> QWALEDFEIGRPLGKGKFGNVYLAREKQSKFILALKVLFKAQLEKAGVEHQLRREVEIQSHLRHPNILRLYGYFHDATRVYLILEYAPLGTVYRELQKLSKFDEQRTATYITELANALSYCHSKRVIHRDIKPENLLLGSAGELKIADFGWSVHAPSSRRTTLAGTLDYLPPEMIEGRMHDEKVDLWSLGVLCYEFLVGKPPFEANTYQETYKRISRVEFTFPDFVTEGARDLISRLLKHNPSQRPMLREVLEHPWITA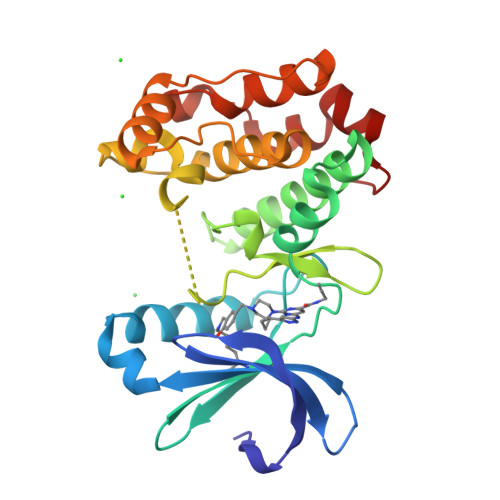NSSKPS> MSILFSSILFSIATFFSRILGLFRDVLFAKYFGVSYELDAYFIAIMFPFFLRKVFGEGAMSSAFVPLYSEKSGEEKDKFLSSVINGFSLIILALVILSYFFPELIINLFGAGSSHETKILAKKLLLITSPSIYFIFLWAISYSILNTNNKFFWPALTPSISNITIIIGTFLSTKYGIISPTIGFLIGSILMFFSIIKSIIKHKYYFTIKHFPHFLKLFFPTFMTMVVSQINTVVD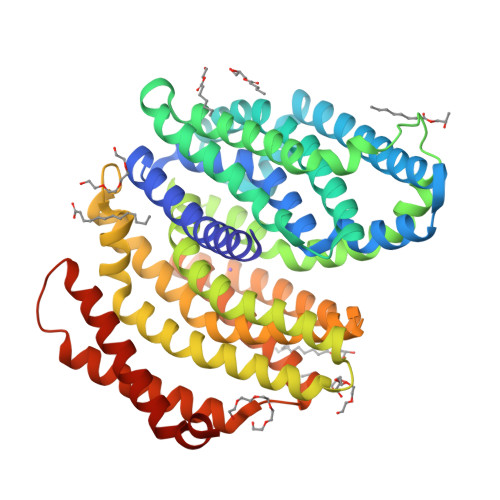MNVVSFYDKGSISYLQYASRFYLLPYGLFAVSVSTVVLSKISNDRKNFNYHLNDALKTTLFFTIPSMVGLIFLSTPIIRFFYEHGAFTSKDTLITSKILIAYTLGLPFYGIYSTISRSYHAIKNTKTPFIAATIVSLSNIILDIIFGLKYGPIGVALATSIAGIIGVLYLLFSVKTFPIKDFLKISLNSLIMLFVIYLTDFTDNEFWFLIQILIGILVYLIFSSIFYRDLIRRFLYARKK Bromodomains (BRDs) are protein interaction modules that specifically recognize ε-N-lysine acetylation motifs, a key event in the reading process of epigenetic marks. The 61 BRDs in the human genome cluster into eight families based on structure/sequence similarity. Despite large sequence variations, all BRD modules share a conserved fold that comprises a left-handed bundle of four α helices (αZ, αA, αB, αC), linked by loop regions of variable length (ZA and BC loops), which line the Kac binding site and determine binding specificity. The four helices form a deep cavity that is extended by the two loop regions (ZA and BC loops), creating a largely hydrophobic Kac binding pocket.

The C and N termini are highly diverse and may comprise additional helices that extend the canonical BRD fold (e.g., the sixth BRD of PB1 has an additional C-terminal helix) or largely extended kinked helices that are present as C- or N-terminal extensions (for instance in TAF1L or ATAD2). A conserved tyrosine (Y97) defines the N terminus of the ZA loop helix present in all BRDs except TRIM28 and the sixth BRD of PB1, which have unusually short ZA loops that have lost this structural element. The most notable structural difference within the BRD core fold is a hairpin insertion located between helix αZ and the ZA loop that is present in all family VIII members. The proximity to the Kac binding site suggests that this insert may play a role in recruitment of acetylated binding partners. In contrast, the second, fourth, fifth, and sixth BRD of PB1, MLL, and TRIM28 interacted with only a few histone Kac peptides.

> SMNVTLLIQELIHNLFVSVMSHQDDEGRCYSDSLAEIPAVDPNFPNKPPLTFDIIRKNVENNRYRRLDLFQEHMFEVLERARRMNRTDSEIYEDAVELQQFFIKIRDELCKNGEILLSPALSYTTKHLHNDVEKERKEKLPKEIEED>MARPLEQAVAAIVCTFQEYAGRCGDKYKLCQAELKEL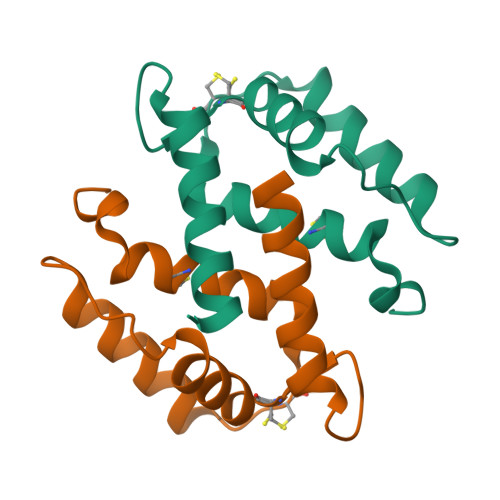LQKELATWTPTEFRECDYNKFMSVLDTNKDCEVDFVEYVRSLACLCLYCHEYFKDCPSEPPCSQ[2x]>HEMNSSKYVESPNYTKVEFGEHYARLRPKKLKANIEYTTPTGHIYRTDHKGRIKEVYVDNLSLKDGDRNSHAQRTVGGEDRLPDDDGGALIARMFGGSKDIDNLVAQSKFINRPFKEKGHWYNLEKEWQEFL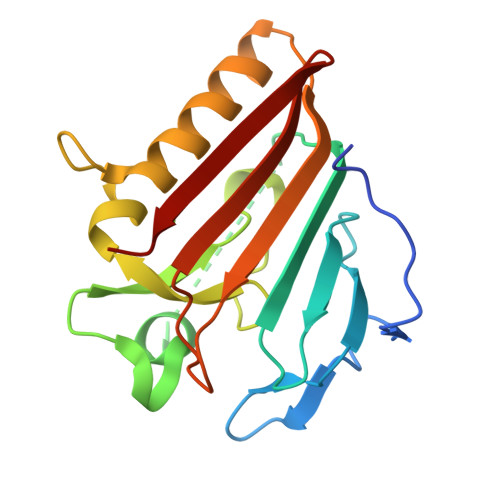NSGKEVKNIKMEVKYSGNSQRPTIFKVEYEINGERNIRRILNK[2x]> SMSFVQHSVRVLQELNKQREKGQYCDATL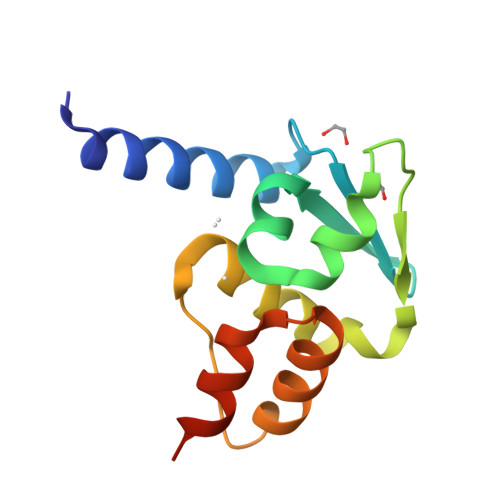DVGGLVFKAHWSVLACCSHFFQSLYGDGSGGSVVLPAGFAEIFGLLLDFFYTGHLALTSGNRDQVLLAARELRVPEAVELCQSFKPKTSV1-{2-deoxy-3,5-O-[phenyl(phosphono)methylidene]-beta-D-threo-pentofuranosyl}-5-[(E)-2-phosphonoethenyl]pyrimidine-2,4(1H,3H)-dione 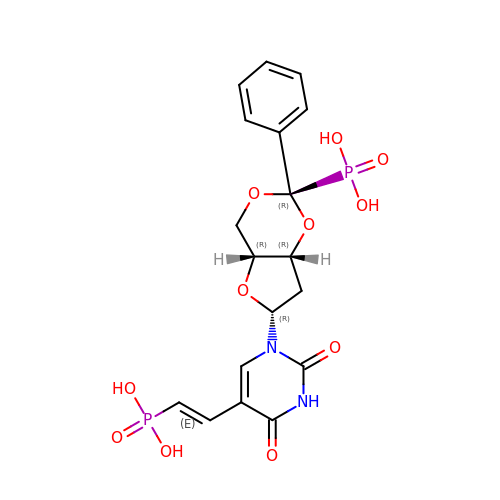| C18 H20 N2 O11 P2 | AYSYVLQGVXZPIY-OAIWFRFLSA-N> ALLV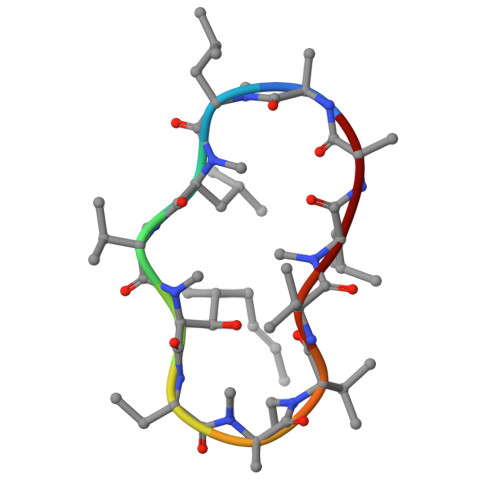TAAXVLA>APQQINDIVHRTITPLIEQQKIPGMAVAVIYQGKPYYFTWGYADIAKKQPVTQQTLFELGSVSKTFTGVLGGDAIARGEIKLSDPTTKYWPELTAKQWNGITLLHLATYTAGGLPLQVPDEVKSSSDLLRFYQNWQPAWAPGTQRLYANSSIGLFGALAVKPSGLSFEQAMQTRVFQPLKLNHTWINVPPAEEKNYAWGYREGKAVHVSPGALDAEAGGVKSTIEDMARWVQSNLKPLDINEKTLQQGIQLAQSRYWQTGDMYQGLGWEMLDW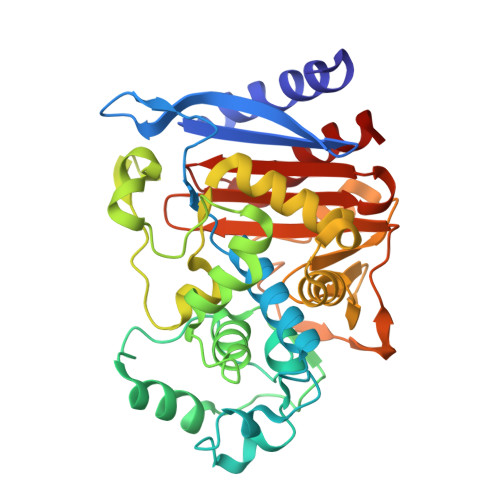PVNPDSIINGSDNKIALAARPVKAITPPTPAVRASWVHKTGATGGFGSYVAFIPEKELGIVMLANKNYPNPARVDAAWQILNALQ[2x]>XSSDPLAVAASIIGILHLI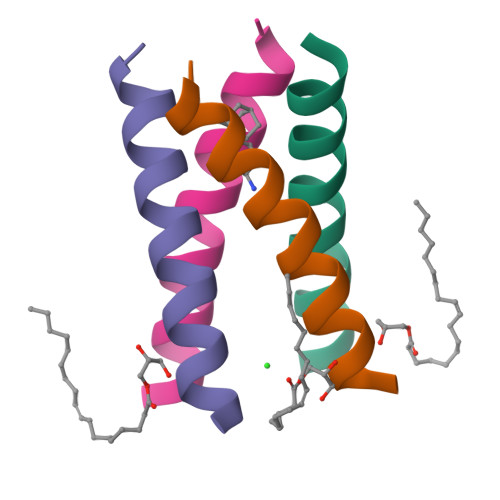LWILDRLX[8x]> SKTNLIVNYLPQNMTQEEFRSLFGSIGEIESCKLVRDKITGQSLGYGFVNYIDP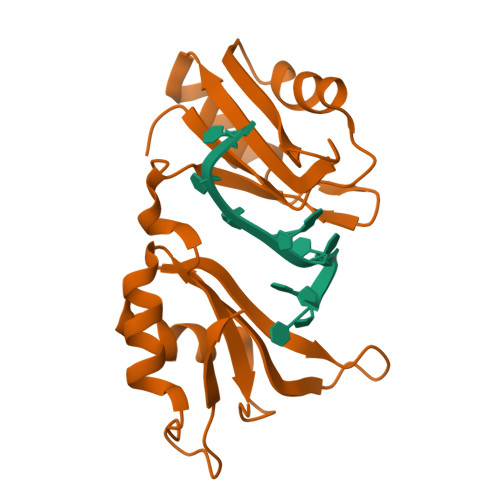KDAEKAINTLNGLRLQTKTIKVSYARPSSASIRDANLYVSGLPKTMTQKELEQLFSQYGRIITSRILVDQVTGVSRGVGFIRFDKRIEAEEAIKGLNGQKPSGATEPITVKFA>[21x]MDQPEAPCSSTGPRLAVARELLLAALEELSQEQLKRFR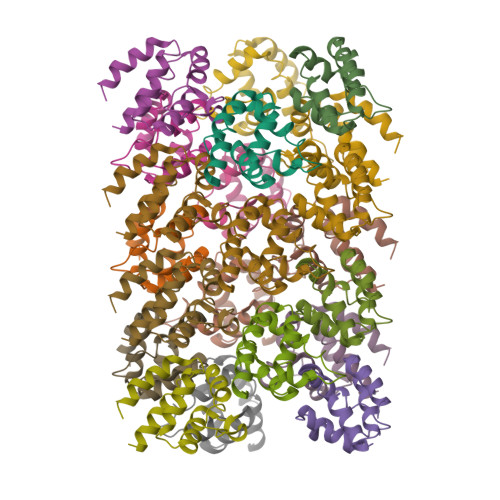HKLRDVGPDGRSIPWGRLERADAVDLAEQLAQFYGPEPALEVARKTLKRADARDVAAQLQERRLQRLG> NDSEVSDPVVVETMKHERILVDHNSALRGAKPINFGY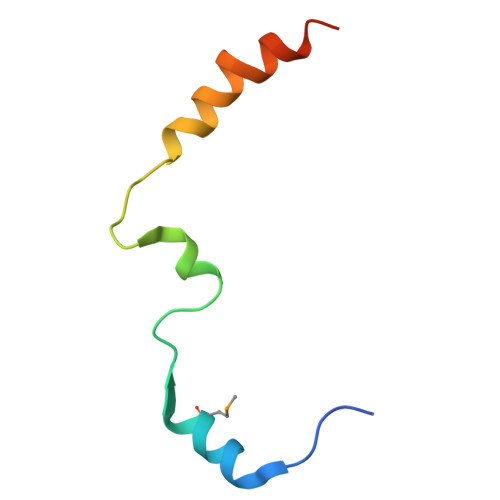LIKDAELKLVQSIKGSLRGS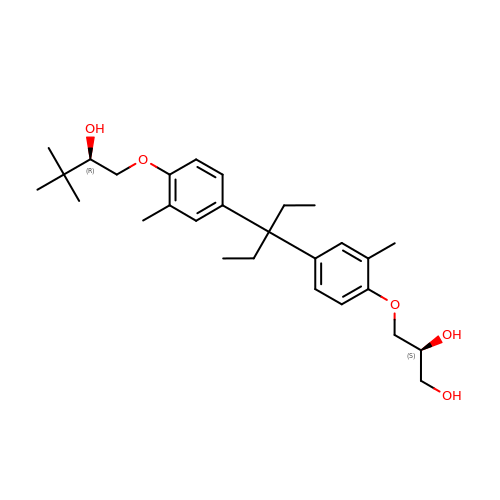(2S)-3-{4-[1-ethyl-1-(4-{[(2R)-2-hydroxy-3,3-dimethylbutyl]oxy}-3-methylphenyl)propyl]-2-methylphenoxy}propane-1,2-diol | C28 H42 O5 | AIKLCYAFOOBGEV-OZXSUGGESA-N The LftR protein transcriptionally regulates the expression of the lmo0980 gene, which encodes a putative multidrug resistance transporter, LieAB (Listerial importer of ethidium bromide as artificial substrate), and facilitates the export of toxic chemicals from the cytoplasm to the extracellular space. LftR contains 108 residues and is expected to belong to the PadR-2 subfamily. As transcriptional regulators, PadR family members commonly contain a winged helix-turn-helix (wHTH) motif to interact with operator DNA. The apparent molecular weights of both LftR proteins were estimated to be 20–24 kDa, whereas the calculated molecular weights are ~12 kDa, indicating that LftR forms a homodimer in solution regardless of construct designs.

The LftRNtH protein was treated with thrombin protease to remove the N-terminal His6 tag, and the tag-free LftR protein (LftRΔNtH) was used for our molecular studies. As a first step in the understanding of LftR at a molecular level, LftRΔNtH and LftRCtH structures were determined and refined at 2.3 and 2.8 Å resolutions, respectively. Although the LftRΔNtH and the LftRCtH structures belong to different space groups (P3221 and P64, respectively), their overall structures are similar and thus the LftRΔNtH structure will be used to describe the structural features of LftR unless otherwise specified. The asymmetric unit of the LftRΔNtH crystal contains two subunits, namely A (residues from -5 to 105; the six N-terminal residues, from -5 to 0, correspond to additional residues that originate from the cloning vector) and B (residues from 3 to 108), which form a homodimer in an isosceles triangle shape. Each LftR subunit consists of five α-helices (H0-H4) and two β-strands (β1 and β2) with a topology of H0 (residues 4–8)–H1 (residues 11–22)–H2 (residues 27–37)–H3 (residues 44–57)–β1 (residues 60–66)–β2 (residues 70–78)–H4 (residues 80–104). LftR dimerization occurs using 25 residues (buried surface area, ~3380 Å2) from the H0, H1, H2, and H4 helices and the H0-H1 loop through numerous intersubunit interactions. Residues 4–8 form an α-helix (H0 helix) in the LftRΔNtH, whereas the corresponding region of LftRCtH adopts an extended coil structure, indicating the flexible nature of the LftR N-terminal residues. As a result, the inter-wHTH distance of the LftRCtH dimer (~81 Å) is ~11 Å longer than that of the LftRΔNtH dimer (~70 Å). The cavity of the LftRCtH dimer structure (cavity surface, ~277 Å2; internal volume, ~148 Å3) is larger than the cavity of the LftRΔNtH dimer (cavity surface, ~157 Å2; internal volume, ~83 Å3) probably due to conformational changes in the dimerization residues. Upon inclusion, the ethidium bromide molecule makes significant clashes with LftRΔNtH cavity residues (residues 9, 10, 11, 89, 93, 96, 97, 100, 4ʹ, 6ʹ, 7ʹ, 8ʹ, 9ʹ, 11ʹ, 15ʹ, 93ʹ, 97ʹ, and 101ʹ) mainly from the H0, H1, and H4 helices of two subunits.

>[2x]GSAKDPMKGLTELLKGSLEGMILERISRGETYGYEITKYLNDLGFDEIVEGTVYTILVRLEKKGLVEIEKKKSELGPPRKFYTLSPAGEEELAIFWKRWDFIQGKIMQVKGGQA>MSPCGYYSKWRNRDRPEYRRNLRFRRFFSSIHPNAAAGSGFNGPGVFITSVTGVWLCFLCIFSMFVTAVVSVSPSSFYESLQVEPTQSEDITRSAHLGDGDEIREAIHKSQDAETKPTFYVCPPPTGSTIVRLEPPRTCPDYHLGKNFTEGIAVVYKENIAAYKFKATVYYKDVIVSTAWAGSSYTQITNRYADRVPIPVSEITDTIDKFGKCSSKATYVRNNHKVEAFNEDKNPQDMPLIASKYNSVGSKAWHTTNDTYMVAGTPGTYRTGTSVNCIIEEVEARSIFPYDSFGLSTGDIIYMSPFFGLRDGAYREHSNYAMDRFHQFEGYRQRDLDTRALLEPAARNFLVTPHLTVGWNWKPKRTEVCSLVKWREVEDVVRDEYAHNFRFTMKTLSTTFISETNEFNLNQIHLSQCVKEEARAIINRIYTTRYNSSHVRTGDIQTYLARGGFVVVFQPLLSNSLARLYLQELVRENTNHSPQKHPTRNTRSRRSVPVELRANRTITTTSSVEFAMLQFTYDHIQEHVNEMLARISSSWCQLQNRERALWSGLFPINPSALASTILDQRVKARILGDVISVSNCPELGSDTRIILQNSMRVSGSTTRCYSRPLISIVSLNGSGTVEGQLGTDNELIMSRDLLEPCVANHKRYFLFGH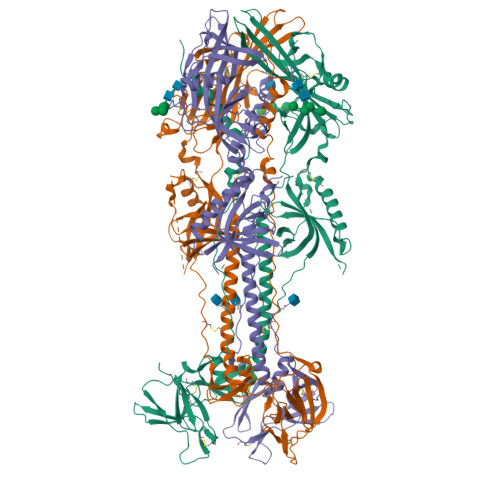HYVYYEDYRYVREIAVHDVGMISTYVDLNLTLLKDREFMPLQVYTRDELRDTGLLDYSEIQRRNQMHSLRFYDIDKVVQYDSGTAIMQGMAQFFQGLGTAGQAVGHVVLGATGALLSTVHGFTTFLSNPFGALAVGLLVLAGLVAAFFAYRYVLKLKTSPMKALYPLTTKGLKQLPEGMDPFAEKPNATDTPIEEIGDSQNTEPSVNSGFDPDKFREAQEMIKYMTLVSAAERQESKARKKNKTSALLTSRLTGLALRNRRGYSRVRTENVTGV[3x]>[2x]GSHMTNTGGRKPDEGERYRAILETAARLICDRGYEGTSMQEIAAACRMTKAGLYHHIQNKEQLLFAIMNYGMDLFEEQVLSRV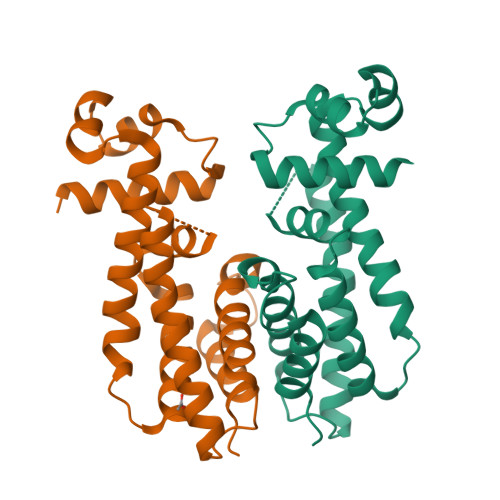QDIANPVERLRACMRHNILLVTRGWSKEVIIILHEHATLTGETRAFIDARKKKYVDFLEEAFSQASQQGLIRPVDPTVGAFSFLGMVLWIYKWFKPDGRLTDEQIADGMVGMLFPPFAAAGDTAGQAGPSPLRMVPSVSATGTDSEDA> MAPTSSIEIVLDKTTASVGEIVTASINIKNITNFSGCQLNMKYDPAVLQPVTSSGVAYTKSTMPGAGTILNSDFNLRQVADNDLEKGILNFSKAYVSLDDYRTAAAPEQTGTVAVVKFKVLKEETSSISFEDTTSVPNAIDGTVLFDWNG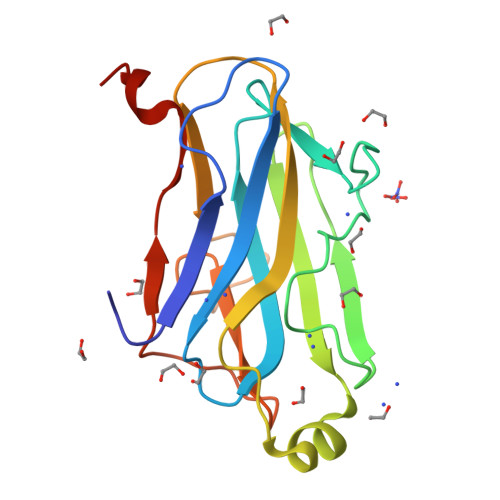DRIQSGYSVIQPAVINLDMIAASLE A potential new target for Chagas' disease chemotherapy is sterol 14α-demethylase (CYP51), a cytochrome P450 heme thiolate-containing enzyme which is involved in biosynthesis of membrane sterols in all biological kingdoms from bacteria to animals. Azoles block CYP51 activity, resulting in decline of the normal complement of endogenous sterols and accumulation of various 14α-methyl sterols with cytostatic or cytoxic consequences. Based upon crystal structures of CYP51 of M. tuberculosis (CYP51Mt), three of the thirteen active site residues, Y76, F83, and H259 (numbering according to CYP51Mt), are invariant throughout the cyp51 gene family. To verify this assumption, we determined the binding modes of second generation compounds containing the N-[4-pyridyl]-formamide moiety by determining their co-crystal structures with CYP51Mt.

Compound 7 was not found in the CYP51Mt active site in the crystal, which is consistent with lack of spectrally detectable binding. Compounds 8 (3-{[(4-methylphenyl)sulfonyl]amino}propylpyridin-4-ylcarbamate), 9 (cis-4-methyl-N-[(1S)-3-(methylsulfanyl)-1-(pyridin-4-ylcarbamoyl)propyl]cyclohexanecarboxamide), and 11 (N-[(1S)-2-methyl-1-(pyridin-4-ylcarbamoyl)propyl]cyclohexanecarboxamide), were observed bound in the CYP51Mt active site as predicted, through the coordination of the heme iron via a lone pair of aromatic nitrogen electrons of the N-[4-pyridyl]-formamide moiety (highlighted in gray in Fig. 2) and interactions with the invariant residues Y76 and H259. Functional groups other than the N-[4-pyridyl]-formamide moiety in compounds 9 and 11 either were accommodated in the species-specific cavity or else protruded through the opening of the active site toward bulk solvent. H259 hydrogen-bonded to the carbonyl oxygen in both compounds, while interactions with Y76 were mediated by two similarly positioned water molecules. The residual Fo-Fc electron density map suggested two alternative conformations for compounds 11 and 9, designated by pink and cyan respectively in Figures 4A and 4B. In the CYP51Mt-compound 9 complex, the methylcyclohexane moiety protruded toward bulk solvent, while the methylsulfanyl group loosely bound in the species-specific cavity in two alternative conformations. The side chain of M433 also adopted two alternative conformations. In both complexes, a portion of the BC-region was disordered and missing from the electron density map. Although racemic mixtures were used for co-crystallization, only one enantiomer of each compound was found in the active site. Compound 9 bound both CYP51Tc and CYP51Tb with the same affinity.

> MSAVALPRVSGGHDEHGHLEEFRTDPIGLMQRVRDELGDVGTFQLAGKQVVLLSGSHANEFFFRAGDDDLDQAKAYPFMTPIFGEGVVFDASPERRKEMLHNAALRGEQMKGHAATIEDQVRRMIADWGEAGEIDLLDFFAELTIYTSSACLIGKKFRDQLDGRFAKLYHELERGTDPLAYVDPYLPIESFRRRDEARNGLVALVADIMNGRIANPPTDKSDRDMLDVLIAVKAETGTPRFSADEITGMFISMMFAGHHTSSGTASWTLIELMRHRDAYAAVIDELDELYGDGRSVSFHALRQIPQLENVLKETLRLHPPLIILMRVAKGEFEVQGHRIHEGDLVAASPAISNRIPEDFPDPHDFVPARYEQPRQEDLLNRWTWIPFGAGRHRCVGAAFAIMQIKAIFSVLLREYEFEMAQPPESYRNDHSKMVVQLAQPAAVRYRRRTGVHHHH> MASVHESLYFNPMMTNGVVHANVFGIKDWVTPYKISVLVLLSEMSKNTKISLVEKRRLNKQILPLLQGPDMTLSKLIKIVEECCPNVSSSVHIRIKLMAEGELKDMEQFFDDL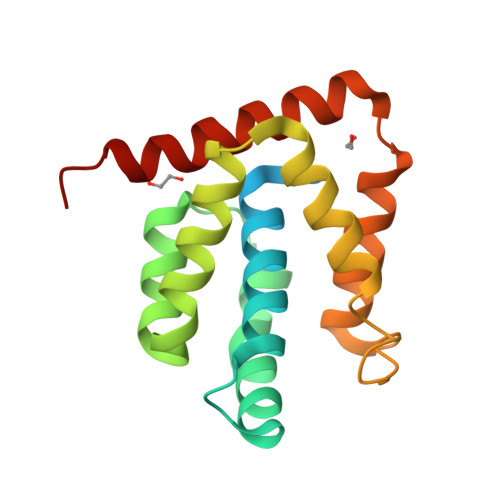ADSFTGTEPEVHKTSVVGLFLRHMILAYNKLSFSQVYKLYTSLQQYFQSDENLYFQ>[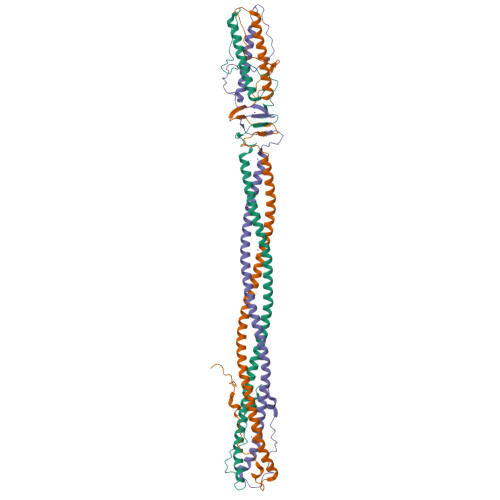6x]GALVPRGSHMADPSLNNPVVIQATRLDASILPRNVFSKSYLLYVIAQGTDVGAIAGKANEAGQGAYDAQVKNDEQDVELADHEARIKQLRIDVDDHESRITANTKAITALNVRVTTAEGEIASLQTNVSALDGRVTTAENNISALQADYVSKTATTSQSLASPLNVTTSYSVGGKKVVGARQTGWTAATGTANKGVFDADLTFAVSDTYTQSEIQAIANALITERRRTKAMEDALRAHGLID>KEWQENKSWNAHFTEHKSQGVVVLWNENKQQGFTNNLKRANQAFLPASTFKIPNSLIALDLGVVKDEHQVFKWDGQTRDIATWNRDHNLITAMKYSVVPVYQEFARQIGEARMSKMLHAFDYGNEDISGNVDSFWLDGGIRISATEQISFLRKLYHNKLHVSERSQRIVKQAMLTEANGDYIIRAKTGYSTRIEPKIGW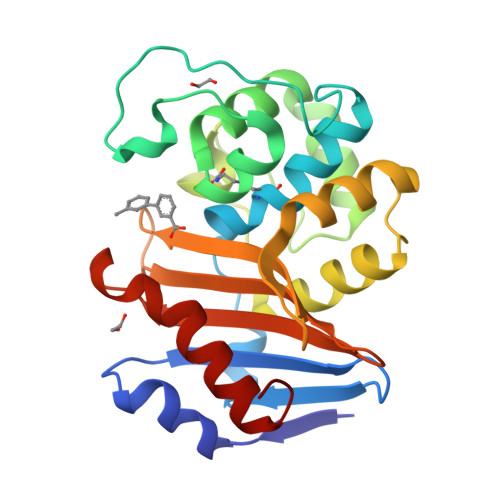WVGWVELDDNVWFFAMNMDMPTSDGLGLRQAITKEVLKQEKIIP[4x]> AATTQIGEIVKTVANTVESEIKAELGVIPSLNAVETGATSNTEPEEAIQTRTVINMHGTAECLVENFLGRSALVCMRSFEYKNHSTSTSSIQKNFFIWTLNTRELVQIRRKMELFTYLRFDTEITIVPTLRLFSSSNVSFSGLPNLTLQAMYVPTGARKPSSQDSFEWQSACNPSVFFKINDPPARLTIPFMSINSAYANFYDGFAGFEKKATVLYG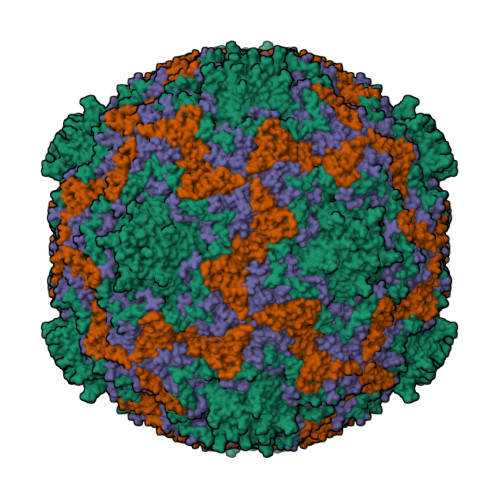INPANTMGNLCLRVVNSYQPVQYTLTVRVYMKPKHIKAWAPRAPRTMPYTNILNNNYAGRSAAPNAPTAIVSHRSTIKTMPNDINLTTA;> SPSAEACGYSDRVLQLKLGNSSIVTQEAANICCAYGEWPTYLPDNEAVAIDKPTQPETSTDRFYTLKSKKWESNSTGWWWKLPDALNQIGMFGQNVQYHYLYRSGFLCHVQCNATKFHQGTLLIVAIPEHQIGKKGTGTSASFAEVMKGAEGGVFEQPYLLDDGTSLACALVYPHQWINLRTNNSATIVLPWMNSAPMDFALRHNNWTLAVIPVCPLAGGTGNTNTYVPITISIAPMCAEYNGLRNAITQ;> GVPTCLLPGSNQFLTTDDHSSAPAFPDFSPTPEMHIPGQVHSMLEIVQIESMMEINNVNDASGVERLRVQISAQSDMDQLLFNIPLDIQLEGPLRNTLLGNISRYYTHWSGSLEMTFMFCGSFMTTGKLIICYTPPGGSSPTDRMQAMLATHVVWDFGLQSSITIIIPWISGSHYRMFNTDAKAINANVGYVTCFMQTNLVAPVGAADQCYIVGMVAAKKDFNLRLMRDSPDIGQSAILPEQA;> GAQVSRQQTGTHENANVATGGSSITYNQINFYKDSYAASASKQDFSQDPSKFTEPVAEALKAGAPVLK> MDVVSLDKPFMYFEEIDNELDYEPESANEVAKKLPYQGQLKLLLGELFFLSKLQRHGILDGATVVYIGSAPGTHIRYLRDHFYNLGVII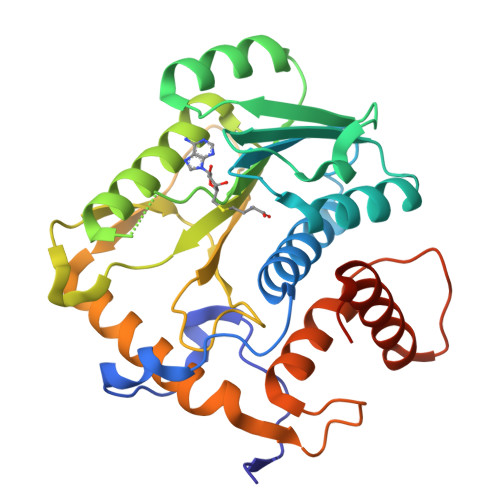KWMLIDGRHHDPILNGLRDVTLVTRFVDEEYLRSIKKQLHPSKIILISDVRSKRGGNEPSTADLLSNYALQNVMISILNPVASSLKWRCPWPDQWIKDFYIPHGNKMLQPFAPSYSAEMRLLSIYTGENMRLTRVTKSDAVNYEKKMYYLNKIVRNKVVVNFDYPNQEYDYFHMYFMLRTVYCNKTFPTTKAKVLFLQQSIFRFLNIPTTSTEKVSHE>MTHHYPTDDIKIKEVKELLPPIAHLYELPISKEASGLVHRTRQEISDLVHGRDKRLLVIIGPCSIHDPKAALEYAERLLKLRKQYENELLIVMRVYFEKPRTTVGWKGLINDPHLDGTFDINFGLSQARSLLLSLNNMGMPASTEFLDMITPQYYADLISWGAIGARTTESQVHRELASGLSCPVGFKNGTDGNLKIAIDAIGAASHSHHFLSVTKAGHSAIVHTGGNPDCHVILRGGKEPNYDAEHVSEAAEQLRAAGVTDKLMIDCSHANSRKDYTRQMEVAQDIAAQLEQDGGNIMGVMVESHLVEGRQDKPEVYGKSITDACIGWGA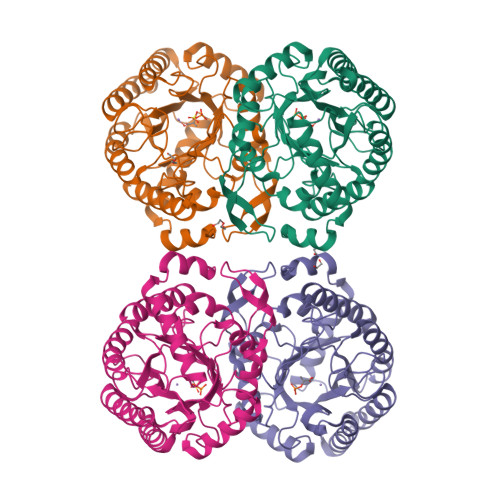TEELLALLAGANKKRMARAS[4x]>AQPTESEKEIYNQVNVVLKDAEGILEDLQSYRGAGHEIR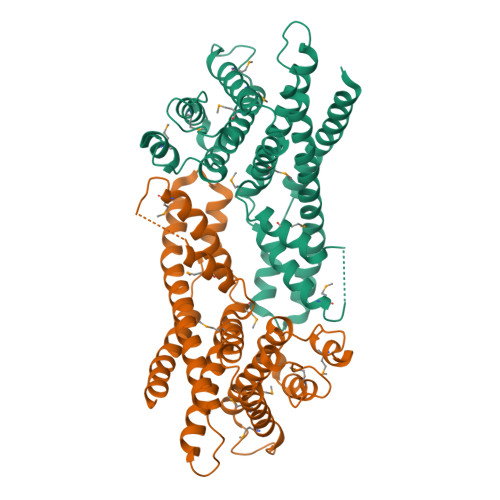EAIQHPADEKLQEKAWGAVVPLVGKLKKFYEFSQRLEAALRGLLGALTSTPYSPTQHLEREQALAKQFAEILHFTLRFDELKMTNPAIQNDFSYYRRTLSRMRINNVPAEGENEVNNELANRMSLFYAEATPMLKTLSDATTKFVSENKNLPIENTTDCLSTMASVCRVMLETPEYRSRFTNEETVSFCLRVMVGVIILYDHVHPVGAFAKTSKIDMKGCIKVLKDQPPNSVEGLLNALRYTTKHLNDETTSKQIRSMLQ[2x]>MGSSHHHHHHSSGLVPRGSRHSTLDFMLGAKADGETILKGLQSIFQEQGMAESVHTWQDHGYLATYTNKNGSFANLRIYPHGLVLLDLQSYDGDAQGKEEIDSILNKVEERMKELSQDSTGRVKRLPPIVRGGAIDRYWPTADGRLVEYDIDEVVYDEDSPYQNIKILHSKQFGNILILSGDVNLAESDLAYTRAIMGSGKEDYTGKDVLILGGGDGGILCEIVKLKPKMVTMVEIDQMVIDGCKKYMRKTCGDVLDNLKGDCYQVLIEDCIPVLKRYAKEGRE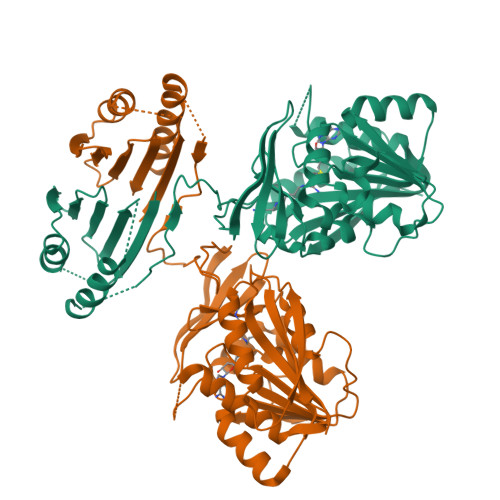FDYVINDLTAVPISTSPEEDSTWEFLRLILDLSMKVLKQDGKYFTQGNCVNLTEALSLYEEQLGRLYCPVEFSKEIVCVPSYLELWVFYTVWKKAKP[4x]> GNSKSGALSKEILEELQLNTKFTEEELSSWYQSFLKECPSGRITRQEFQTIYSKFFPEADPKAYAQHVFRSFDANSDGTLD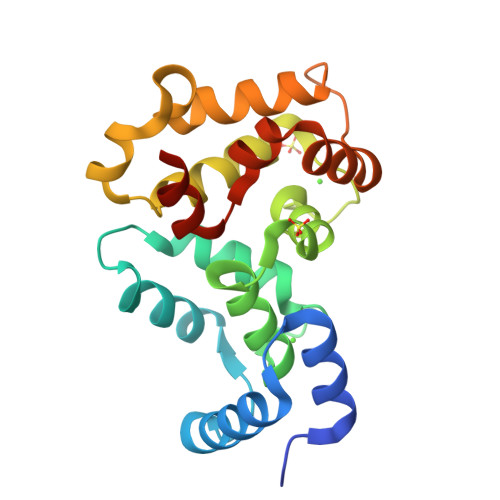FKEYVIALHMTSAGKTNQKLEWAFSLYDVDGNGTISKNEVLEIVTAIFKMISPEDTKHLPEDENTPEKRAAKIWGFFGKKDDDKLTEKEFIEGTLANKEILRLIQFEPQKVKEKLKEKKL>SEDNQRSRFRKICVFCGSHSGHREVFSDAAIELGNELVKRKIDLVYGGGSVGLMGLISRRVYEGGLHVLGIIPKALMPIEISGETVGDVRVVADMHERKAAMAQEAEAFIALPGGYGTMEELLEMITWSQLGIHKKTVGLLNVDGYYNNLLALFDTGVEEGFIKPGARNIVVSAPTAKELMEKMEEYTPSHMHVASHESWKVEELGD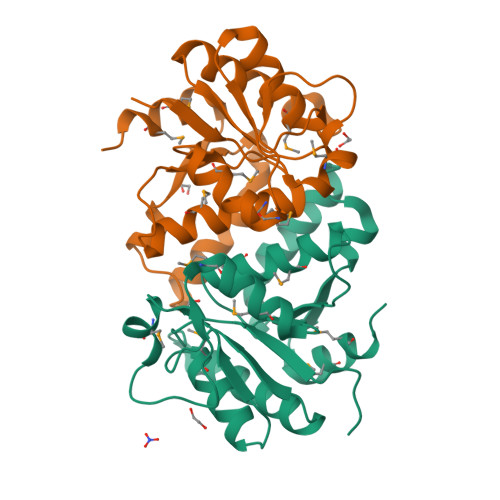YPGQENKPQ[2x]>[2x]MRGSTDPFELVDIPKISYNPSELSEPRFLEYSNLSDKLHLREAIDKILIPRVVGTTNH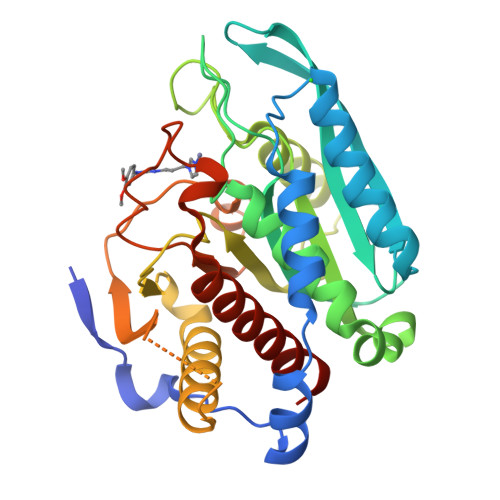SIVREYIVQSLRDLDWDVEVNSFHDHAPIKGKLHFHNIIATLNPNAERYLVLSCHYDSKYMPGVEFLGATDSAVPCAMLLNLAQVLQEQLKPLKKSKLSLMLLFFDGEEAFEEWGPKDSIYGARHLAKKWHHEGKLDRIDMLVLLDLLGAPDPAFYSFFENTESWYMRIQSVETRLAKLQLLERYASSGVAQRDPTRYFQSQAMRSSFIEDDHIPFLRRNVPILHLIPVPFPSVWHTPDDNASVIDYATTDNLALIIRLFALEYLLAGTEAK> M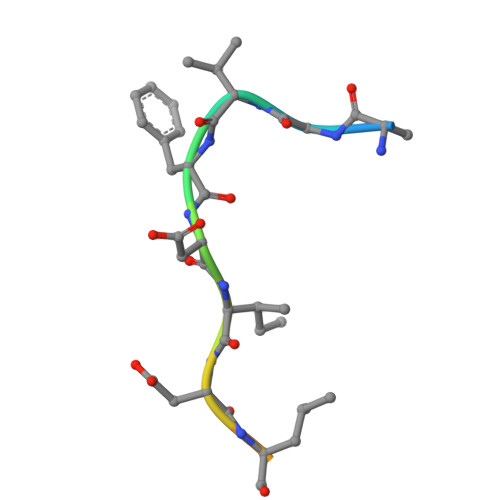AGVFDIDLDQPED>[3x]GSHMSQATSQPINFQVQKDGSSEKSHMDDYMQHPGKVIKQNNKYYFQTVLNNASFWKEYKFYNANNQELATTVVNDNKKADTRTINVAVEPGYKSLTTKVHIVVPQINANHRYTTHLEFE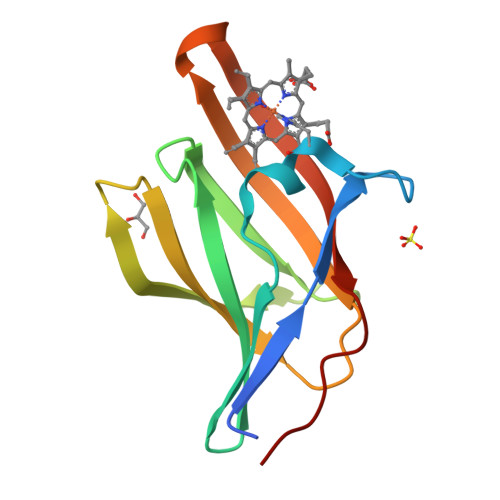KAIPTLA4-[[1,1-bis(oxidanylidene)-7-propan-2-yl-4~{H}-1$l^{6},2,4-benzothiadiazin-3-yl]amino]benzoic acid | C17 H17 N3 O4 S | 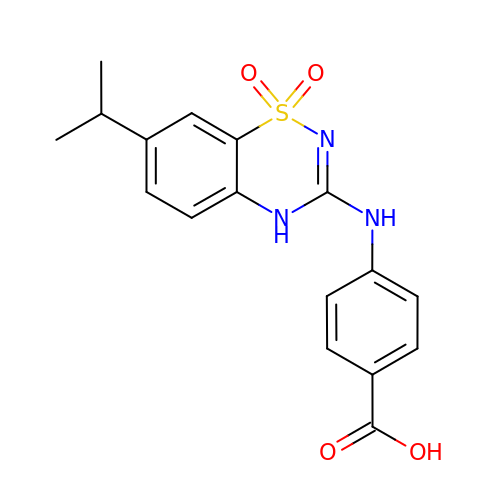XHDRFBQZXYWJHC-UHFFFAOYSA-N>[12x]RAELNQGLIDFLKASPTPFHATASLARRLEAAGYRRLDERDAWHTETGGRYYVTRNDSSLIAIRLGRRSPLESGFRLVGAHTDSPCLRVKPNPEIARNGFLQLGVEVYGGALFAPWFDRDLSLAGRVTFRANGKLESRLVDFRKAIAVIPNLNIHLNRAANEGWPINAQNELPPIIAQLAPGEAADFR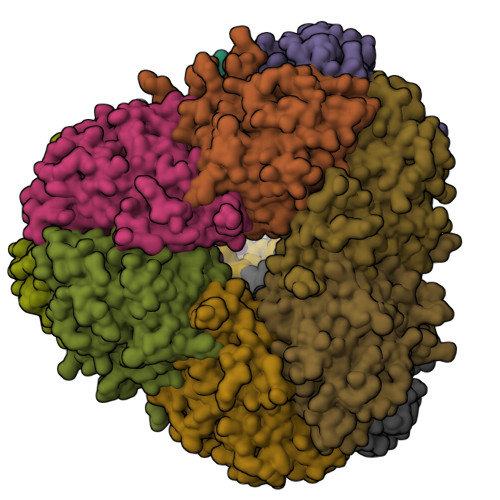LLLDEQLLREHGITADVVLDYELSFYDTQSAAVVGLNDEFIAGARLDNLLSCHAGLEALLNAEGDENCILVCTDHEEVGSCSHCGADGPFLEQVLRRLLPEGDAFSRAIQRSLLVSADNAHGVHPNYADRHDANHGPALNGGPVIKINSNQRYATNSETAGFFRHLCQDSEVPVQSFVTRSDMGCGSTIGPITASQVGVRTVDIGLPTFAMHSIRELAGSHDLAHLVKVLGAFYASSELP> ISIMDRSEIVARENPVITQRVTNLLQTNAPLLFMPIDIHEVRYGAYTLFMYGSLENGYKAEVRIENIPVFFDVQIEFNDTNQLFLKSLLTAENIVYERLETLTQRPVMGYREKEKEFAPYIRIFFKSLYERRKAITYLNNMGYNTAADDTTCYYRMVSRELKLPLTSWIQLQHYSYEPRGLVHRFSVTPEDLVSYQNDGPTDHSIVMAYDIETYSPVKGTVPDPNQANDVVFMICMRIFWIHSTEPLASTCITMAPCKKSSEWTTILCSSEKNLLLSFAEQFSRWAPDICTGFNDSRYDWPFIVEKSMQHGILEEIFNKMSLFWHQKLDTILKCYYVKEKRVKISAEKSIISSFLHTPGCLPIDVRNMCMQLYPKAEKTSLKAFLENCGLDSKVDLPYHLMWKYYETRDSEKIADVAYYCIIDAQRCQDLLVRHNVIPDRREVGILSYTSLYDCIYYAGGHKVCNMLIAYAIHDEYGRIACSTIARGKREHGKYPGAFVIDPVKGLEQDKPTTGLDFASLYPSLIMAYNFS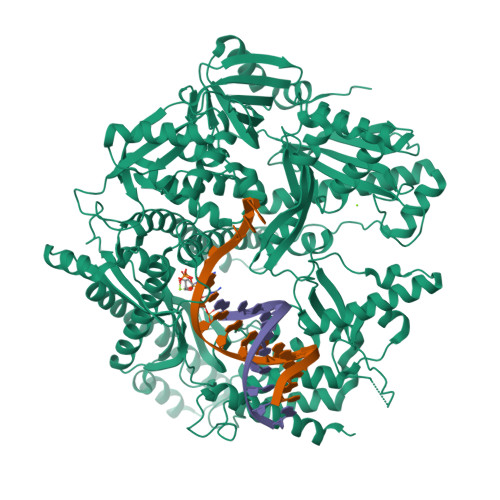PEKFVASRDEANSLMAKGESLHYVSFHFNNRLVEGWFVWHNNVPDKMGLYPKVLIDLLNKRTALKQELKKLGEKKECIHESHPGFKELQFRHAMVDAKQKALKIFMNTFYGEAGNNLSPFFLLPLAGGVTSSGQYNLKLVYNFVINKGYGIKYGDTDSLYITCPDSLYTEVTDAYLNSQKTIKHYEQLCHEKVLLSMKAMSTLCAEVNEYLRQDNGTSYLRMAYEEVLFPVCFTGKKKYYGIAHVNTPNFNTKELFIRGIDIIKQGQTKLTKTIGTRIMEESMKLRRPEDHRPPLIEIVKTVLKDAVVNMKQWNFEDFIQTDAWRPDKDNKAVQIFMSRMHARREQLKKHGAAASQFAEPEPGERFSYVIVEKQVQFDIQGHRTDSSRKGDKMEYVSEAKAKNLPIDILFYINNYVLGLCARFINENEEFQPPDNVSNKDEYAQRRAKSYLQKFVQSIHPK> GPMGSLRNVAKIVEQIDRAVYSIDLAIYTFTSLFLADSIKRALQRGVIIRIISDGEMVYSKGSQISMLAQLGVPVRVPITTNLMHNKFCIIDGFERVEEIRLLRKLKFMRPCYSIVISGSVNWTALGLGGNWENCIITADDKLTATFQA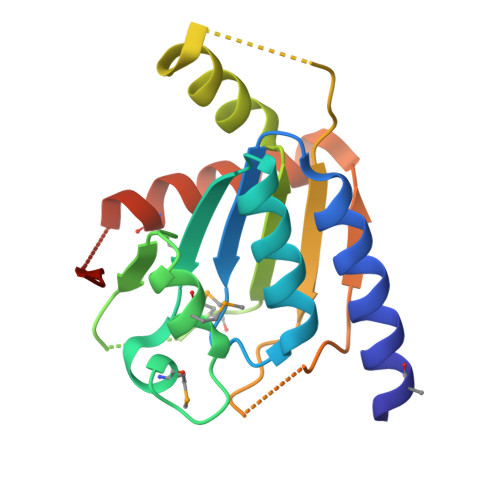EFQRMWRAFAKTEGSQIQLK>[8x]AMMKAAVVRAFGAPLTIDEVPVPQPGPGQVQVKIEASGVCHTDLHAADGDWP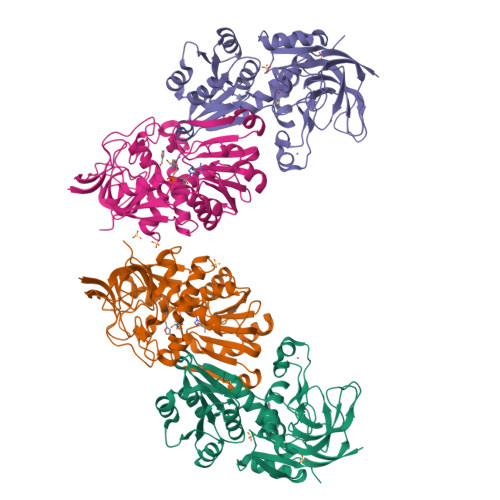VKPTLPFIPGHEGVGYVSAVGSGVSRVKEGDRVGVPWLYSACGYCEHCLQGWETLCEKQQNTGYSVNGGYGEYVVADPNYVGLLPDKVGFVEIAPILCAGVTVYKGLKVTDTRPGQWVVISGIGGLGHVAVQYARAMGLRVAAVDIDDAKLNLARRLGAEVAVNARDTDPAAWLQKEIGGAHGVLVTAVSPKAFSQAIGMVRRGGTIALNGLPPGDFGTPIFDVVLKGITIRGSIVGTRSDLQESLDFAAHGDVKATVSTAKLDDVNDVFGRLREGKVEGRVVLDFSR>[2x]SLSCRPPMVKLVCPADNLRAEGLECTKTCQNYDLECMSMGCVSGCLCPPGMVRHENRCVALERCPCFHQGKEYAPGETVKIGCNTCVCRDRKWNCTDHVCDATCSTIGMAHYLTFDGLKYLFPGECQYVLVQDYCGSNPGTFRILVGNKG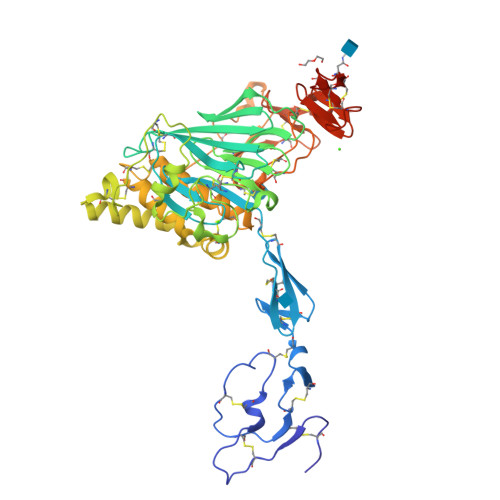CSHPSVKCKKRVTILVEGGEIELFDGEVNVKRPMKDETHFEVVESGRYIILLLGKALSVVWDRHLSISVVLKQTYQEKVCGLCGNFDGIQNNDLTSSNLQVEEDPVDFGNSWKVSSQCADTRKVPLDSSPATCHNNIMKQTMVDSSCRILTSDVFQDCNKLVDPEPYLDVCIYDTCSCESIGDCAAFCDTIAAYAHVCAQHGKVVTWRTATLCPQSCEERNLRENGYEAEWRYNSCAPACQVTCQHPEPLACPVQCVEGCHAHCPPGKILDELLQTCVDPEDCPVCEVAGRRFASGKKVTLNPSDPEHCQICHCDVVNLTCEACQEPGGLVPR>[2x]AGKPVLHYFNARGRMECIRWLLAAAGVEFEEKFIQSPEDLEKLKKDGNLMFDQVPMVEIDGMKLAQTRAILNYIATKYDLYGKDMKERALI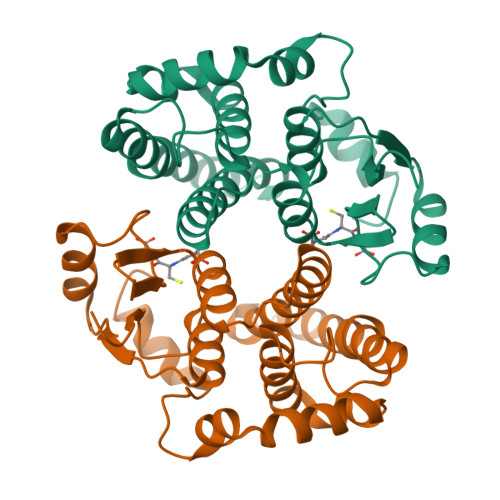DMYSEGILDLTEMIGQLVLCPPDQREAKTALAKDRTKNRYLPAFEKVLKSHGQDYLVGNRLTRVDIHLLEVLLYVEEFDASLLTPFPLLKAFKSRISSLPNVKKFLQPGSQRKPPMDAKQIQEARKAFKIQ> X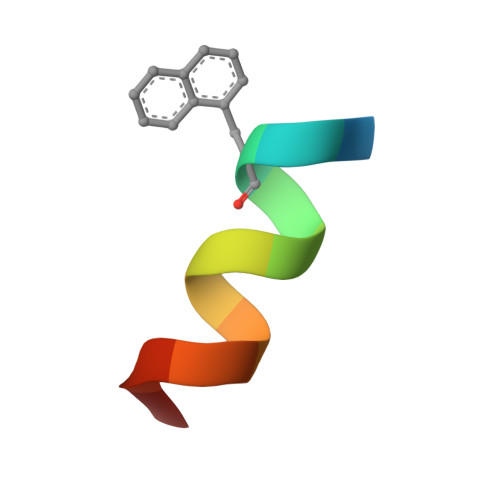EKAARLARRIAX> MEAD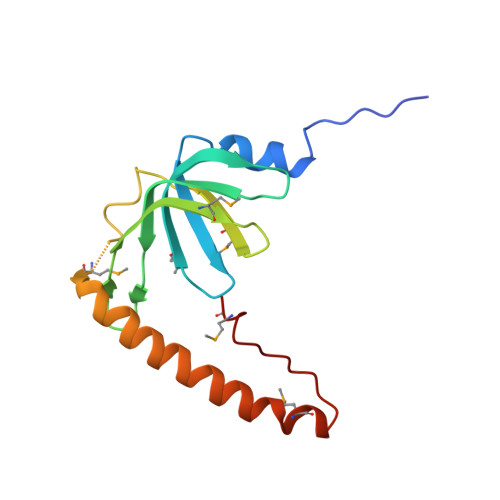LYLDQYNFTTTAAIVSSVDRKIFVLLRDGRMLFGVLRTFDQYANLILQDCVERIYFSEENKYAEEDRGIFMIRGENVVMLGEVDIDKEDQPLEAMERIPFKEAWLTKQKNDEKRFKEETHKGKKMARHGIVYDFHKSDMY N-{[3-(4-amino-2-chloroquinazolin-7-yl)phenyl]sulfonyl}-L-threoninamide 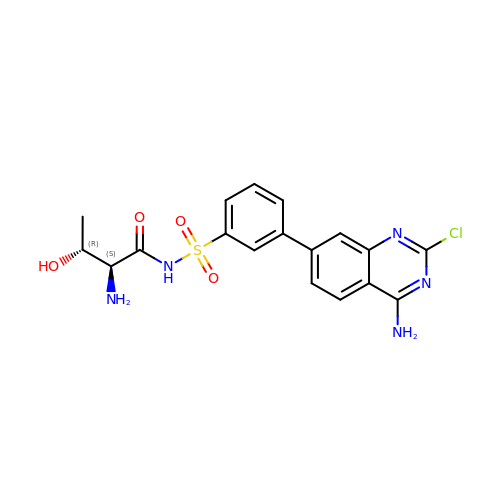| C18 H18 Cl N5 O4 S | MSFGWBJSNPMREF-PSLIRLAXSA-N> MTRLDSVERAVADIAAGKAVIVIDDEDRENEGDLIFAAEKATPEMVAFMVRYTSGYLCVPLDGAICDRLGLLPMYAVNQDKHGTAYTVTVDARNGIGTGISASDRATTMRLLAD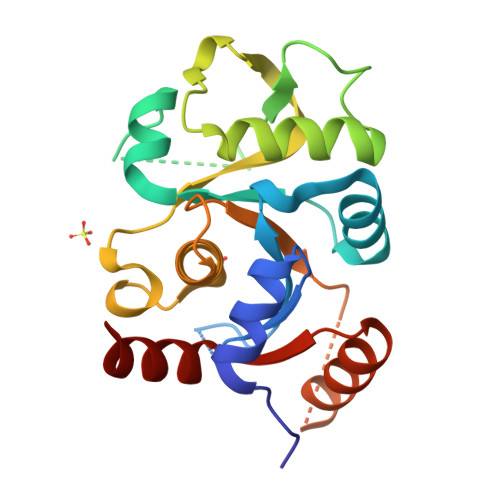PTSVADDFTRPGHVVPLRAKDGGVLRRPGHTEAAVDLARMAGLQPAGAICEIVSQKDEGSMAHTDELRVFADEHGLALITIADLIEWRRKHE> MTYWICITNRENWEVIK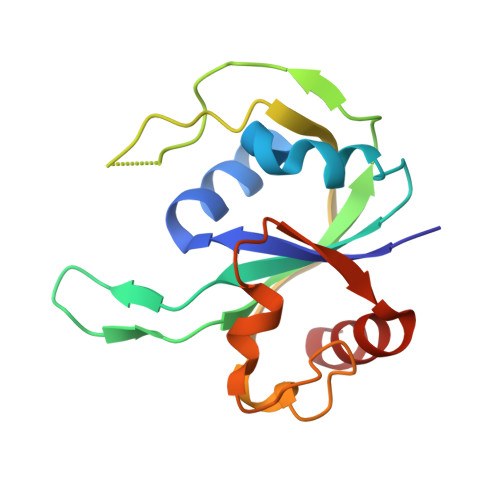RHNVWGVPKKHKNTLSRVKPGDKLVIYVRQEKDKEGNLLEPKIVGIYEVTSEPYVDFSRIFKPHRGGKETYPYRVKIKPIKIGEINFKPLINDLKFIKNKKRWSMHFFGKAMRELPEEDYKLIEKLLL> SGWRAPSCTKVTGD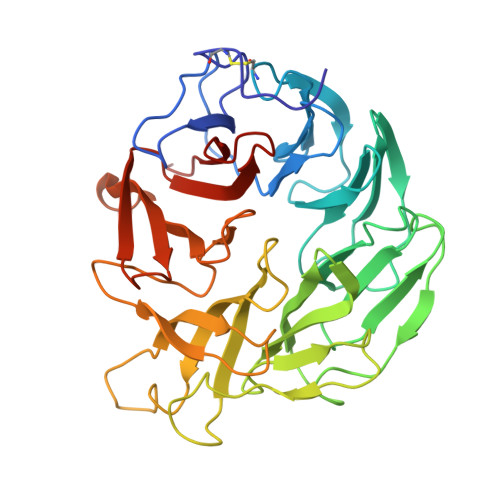GAVTFTTDDGATLAPTTGTLQSVSYTHGLVALDTPNTLLATHNDELQRSTDAGCTWTKVATLGSGSTWLTAATGGRAFAWEKNGGYLARVDGRTVTKLSSPSADIVGVGTDKARRDHVRLAGSDGQLYDSTDAGATWKPLGKLAFGPGASVYTVSFDPADLDHAVAGGMTTGGAVTTDGGATWTAATGLSATAGGKSNLFAASVSPADRNVVYALGIDLVEAAPNSGAEGRHLYRSTDGGRTYTRIVDDTPDTELTNSTLLAPSPVDPNVLYFEYGTYFQAYGTDLYRYDARTGKVGKTHNAHDGISAIAFNPARPSVMYLGLEEVQI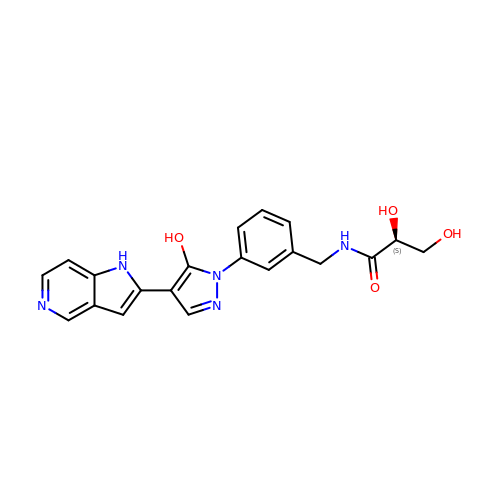(2S)-2,3-dihydroxy-N-[[3-[5-hydroxy-4-(1H-pyrrolo[3,2-c]pyridin-2-yl)pyrazol-1-yl]phenyl]methyl]propanamide | C20 H19 N5 O4 | RWODSWBBNXCAKK-SFHVURJKSA-N> SMSPAYLKEILEQLLEAIVVATNPSGRLISELFQKLPSKVQYPDYYAIIKEPIDLKTIAQRIQNGSYKSIHAMAKDIDLLAKNAKTYNE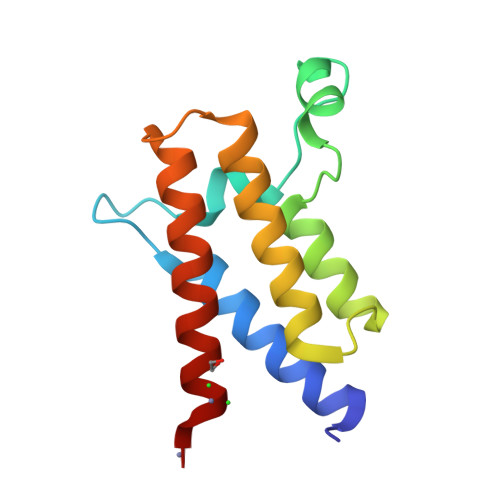PGSQVFKDANSIKKIFYMKKAEIEHHE>[2x]MGHHHHHHSIVKTMIVDDSAFMRNILKRILSTTNKYVVIGEAANGADAIKMAEELQPDLISMDIVMPETDGITATKAIKEKTPEIKIVMCTSVDQEQKMIDAVNAGADGYIVKPFQAPKILEQFNKLFPVLFQGPSAGLVPR;>GSGGIEGGSMGTIKS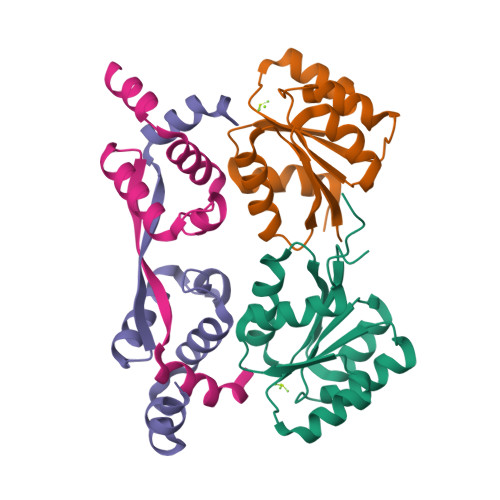LLPKSEDDLDSEMAVESWSGDKLKNEVEQLAPEEQEILTAIYTGITSLELPGMMGMDIDEVEKVLEKLIDQGFLDLVRIRKETDLTEKGRAVTNFIITNF[2x]>WTGRQKARGAATRARQKQRASLETMDKAVQRFRLQNPDLDSEALLTLPLLQLVQKLQSGELSPEAVFFTYLGKAWEV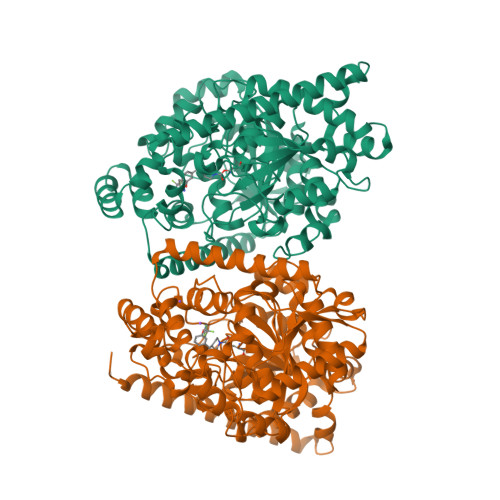NKGTNCVTSYLTDCETQLSQAPRQGLLYGVPVSLKECFSYKGHDSTLGLSLNEGMPSESDCVVVQVLKLQGAVPFVHTNVPQSMFSYDCSNPLFGQTMNPWKSSKSPGGSSGGEGALIGSGGSPLGLGTDIGGSIRFPSAFCGICGLKPTGNRLSKSGLKGCVYGQTAVQLSLGPMARDVESLALCLKALLCEHLFTLDPTVPPLPFREEVYRSSRPLRVGYYETDNYTMPSPAMRRALIETKQRLEAAGHTLIPFLPNNIPYALEVLSTGGLFSDGGRSFLQNFKGDFVDPCLGDLILILRLPSWFKRLLSLLLKPLFPRLAAFLNNMRPRSAEKLWKLQHEIEMYRQSVIAQWKAMNLDVLLTPMLGPALDLNTPGRATGAVSYTMLYNCLDFPAGVVPVTTVTAEDDAQMELYKGYFGDIWDIILKKAMKNSVGLPVAVQCVALPWQEELCLRFMREVEQLMT[2x]> IRCFITPDITSKDCPNGHVCYTKTWCDAFCSIRGKRVD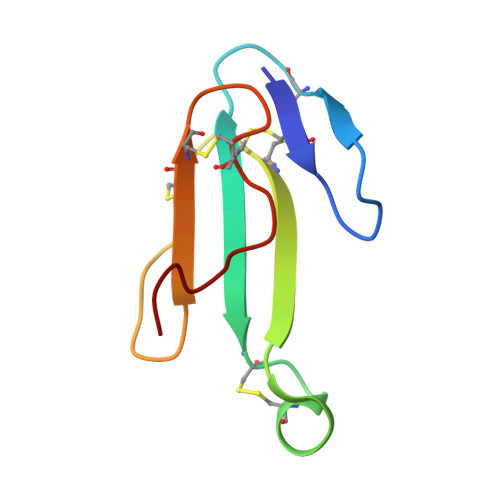LGCAATCPTVKTGVDIQCCSTDNCNPFPTRKRP> KTFTRCGLVHELRKHGFEENLMRNWVCLVEHESSRDTSKTNTNRNGSKDYGLFQINDRYWCSKGAS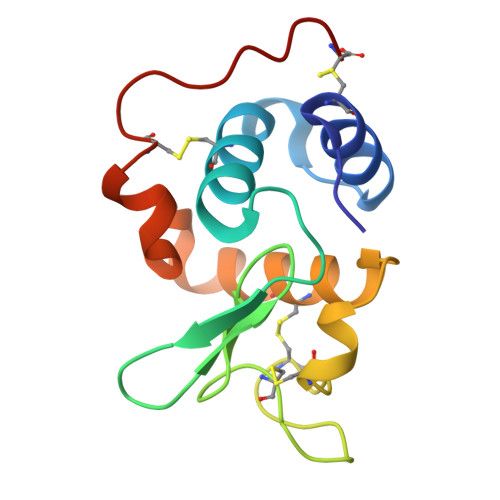PGKDCNVKCSDLLTDDITKAAKCAKKIYKRHRFDAWYGWKNHCQGSLPDISSC> GPLGSADTLERVTKIIVDRLGVDEADVKLEASFKEDLGADXLDVVELVMELED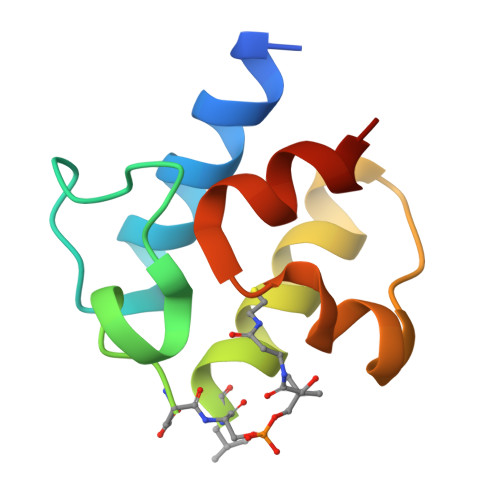EFDMEISDEDAEKIATVGDAVNYIQNQQ>MKTKKHAL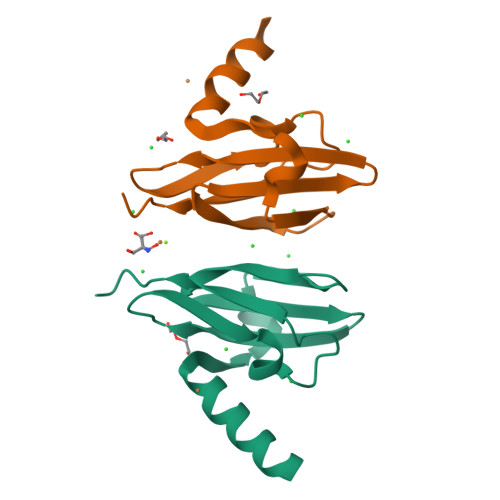LFAALLLGGMSASYALEMTGLKPGVPASTATAQAMAKRHATLYGDPAGQSQASRIIDVKPGMRYVNVDSGETVAFRAGEKIVAWTFAQMVRDTSVDLGLLMPDLPGSAGVRVYIDRSDLFTGG[2x]>[2x]ESQFLKEELVAAVEDVRKQGDLMKAAAGEFADDPCSSVKRGNMVRAARALLSAVTRLLILADMADVYKLLVQLKVVEDGILKLRNAGNEQDLGIQYKALKPEVDKLNIMAAKRQQE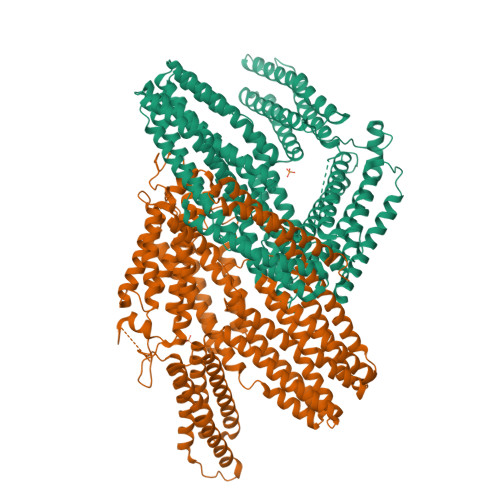LKDVGHRDQMAAARGILQKNVPILYTASQACLQHPDVAAYKANRDLIYKQLQQAVTGISNAAQATASDDASQHQGGGGGELAYALNNFDKQIIVDPLSFSEERFRPSLEERLESIISGAALMADSSCTRDDRRERIVAECNAVRQALQDLLSEYMGNAGRKERSDALNSAIDKMTKKTRDLRRQLRKAVMDHVSDSFLETNVPLLVLIEAAKNGNEKEVKEYAQVFREHANKLIEVANLACSISNNEEGVKLVRMSASQLEALCPQVINAALALAAKPQSKLAQENMDLFKEQWEKQVRVLTDAVDDITSIDDFLAVSENHILEDVNKCVIALQEKDVDGLDRTAGAIRGRAARVIHVVTSEMDNYEPGVYTEKVLEATKLLSNTVMPRFTEQVEAAVEALSSDPAQPMDENEFIDASRLVYDGIRDIRKAVLMIRTPEELDDSDFETEDFDVRSRTSVQTEDDQLIAGQSARAIMAQLPQEQKAKIAEQVASFQEEKSKLDAEVSKWDDSGNDIIVLAKQMCMIMMEMTDFTRGKGPLKNTSDVISAAKKIAEAGSRMDKLGRTIADHCPDSACKQDLLAYLQRIALYCHQLNICSKVKAEVQNLGGELVVSGVDSAMSLIQAAKNLMNAVVQTVKASYVASTKYQKSQGMASLNLPAVSWKMKAPEKKPLVKREKQDETQTKIKRASQKKHVNPVQALSEFKAMDSIPHHHHHH> KNVSGSVKLWVDTTQVPYYKKIVANFNKKYPDVKVKVTQSPNGSANAKTDVGKDPAKAADVFEVANDQLGSMAEAGYINPLSPDATKAVKNNNVAVASEGVTWKGKMFAYPFAEQAQTIYYNKSKLTADDVKTWDGLTAKGVLATDFTNAYNFYPVFLSAGTQLYGKTGETVKGTDVNSAKGEQAMAWFAQQKSNKGVMQTSNALNQLKSGKAAAILDGPWNSANIKKILGKNFAVAPYPTIKLDGKDVQMQAFLGIETFAVNSHASGSNQKA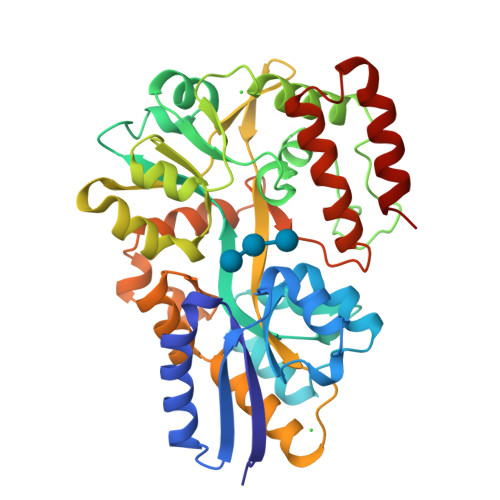AATLASFITNKESQLIVYDHSGQIPVDKTAQKSSKVASDPVAGAVMTMAKPGNSTLMPKMPQMATFWNDAAPLINGAYTGSIPASQYSTKLDTFVKNISKAN> MSQSNRELVVDFLS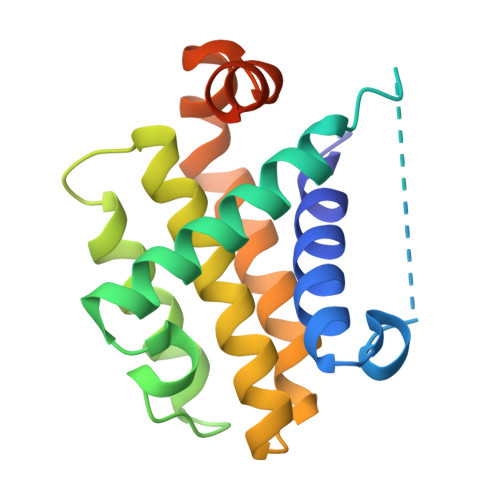YKLSQKGYSWSQFSDVEENRTEAPEGTESEMAAVKQALREAGDEFELRYRRAFSDLTSQLHITPGTAYQSFEQVVNELFRDGVNWGRIVAFFSFGGALCVESVDKEMQVLVSRIAAWMATYLNDHLEPWIQENGGWDTFVELYGNNAAAESRKGQER>[2x]MKANLLCGNRNLPKHILVEHKHEHWIGIDRGTLILLESGITPQFAVGDFDSISDSERNFIQQQIEINPYNSEKDDTDLALG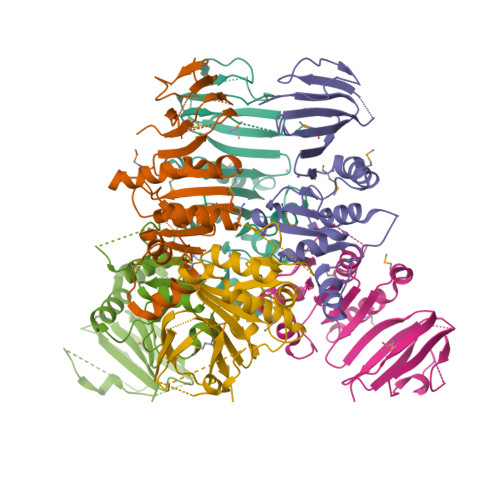IDQAVKRGYRNIDVYGATGGRLDHFMGALQILEKPEYAKMNINIKLIDDTNEIQFIQKGQFNVTYSEQFPYISFIPVIYPTVISLKGFKYNLQNETLKLGSTLTISNELSQSCGNIEIIEGSVLMIRSKDE2-[1-(cyclohexylmethyl)piperidin-4-yl]-1-{3-[3-{[2-(piperidin-1-yl)ethyl]sulfanyl}-4-(trifluoromethyl)phenyl]-1-propyl-1,4,6,7-tetrahydro-5H-pyrazolo[4,3-c]pyridin-5-yl}ethan-1-one | C37 H54 F3 N5 O S | 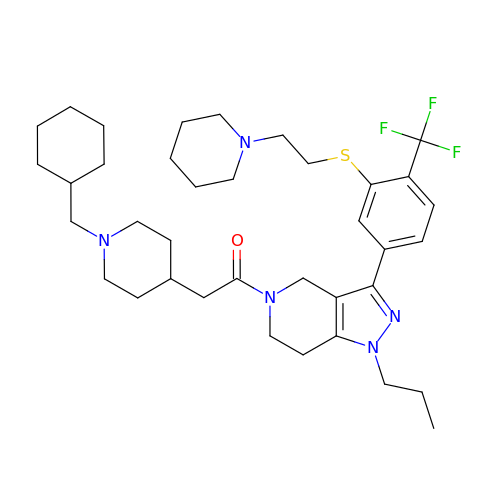QKTCJJYONPZDQD-UHFFFAOYSA-N> MWNKAVIGDVNADGVVNISDYVLMKRYILRIIADFPADDDMWVGDVNGDNVINDIDCNYLKRYLLHMIREFPKNSYNSA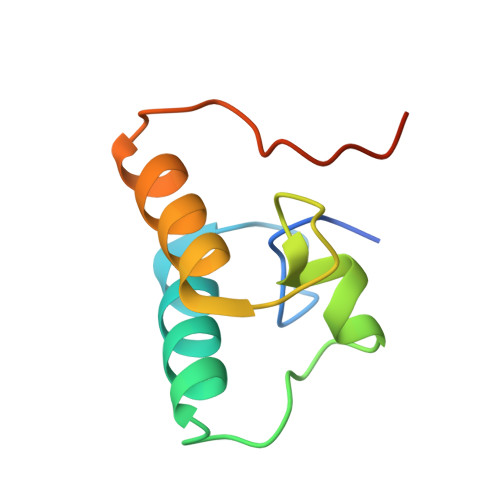PTF>[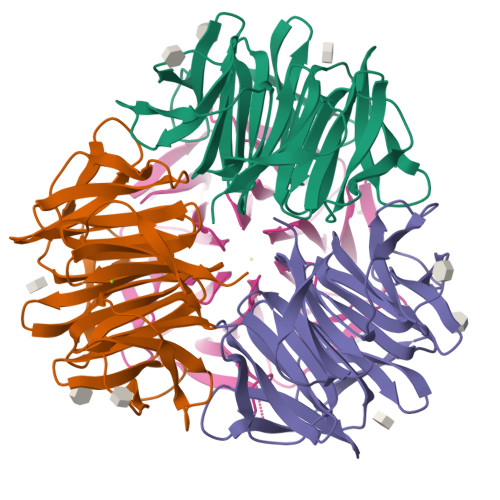2x]MPWKGISGSLSRISAGSVTNVWGVNAANNIYRYTGDDAKPWVQIPGALTDIGAAADGTVWGVNAAGNIYRYVWDSNHWTQIKGALKRISAGSRTNVWGVNAGGAIYRYTGDDANPWVQIPGVLSDIGAGADGTVWGVNAAGEIYRYTGDQGDPNHWVKIPGALSAISAGIKTNVWGVNSANNIYTSTGDDKNPWLGIGGSLVDIGAGTDGVVWGVNAGGGIYRWIRD>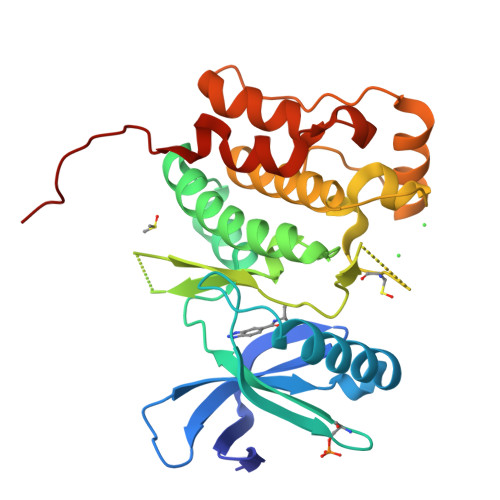 SLGGTETVGKFEFSRKDLIGHGAFAVVFKGRHREKHDLEVAVKCINKKNLAKSQTLLGKEIKILKELKHENIVALYDFQEMANSVYLVMEYCNGGDLADYLHAMRTLSEDTIRLFLQQIAGAMRLLHSKGIIHRDLKPQNILLSNPAGRRANPNSIRVKIADFGFARYLQSNMMAATLCGSPMYMAPEVIMAQHYDGKADLWSIGTIVYQCLTGKAPFQAASPQDLRLFYEKNKTLVPTIPRETSAPLRQLLLALLQRNHKDRMDFDEFFHHPFLDASPSVRKSPPV> TRDQNGTWEMESNENFEGYMKALDIDFCTRKIAVRCTQTKVIDQDGDNFKDKTTSTHRNYDVDF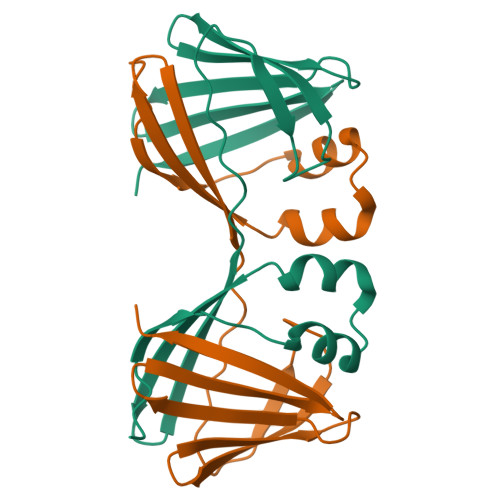TVGVEFDEYTKSLDNRHVKALVTWEGDVLVCVQKGEKENRGWKKWIEGDKLYLELTCGDQVCRQVFKKK>[3x]QAEEWYFGKITRRESERLLLNP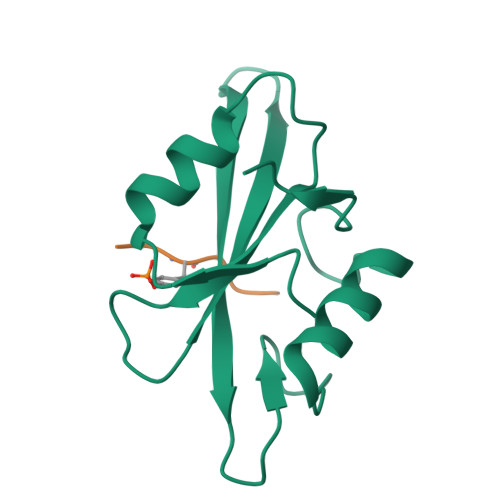ENPRGTFLVRESETTKGAYCLSVSDFDNAKGLNVKHYKIRKLDSGGFYITSRTQFSSLQQLVAYYSKHADGLCHRLTNVCPT;>[3x]EPQYEEIPIYL> SSVVVDTNGQPVSNGADAYYLVPVSHGHAGLALAKIGNEAEPRAVVLDPHHRPGLPVRFESPLRINIIKESYFLNIKFGPSSSDSGVWDVI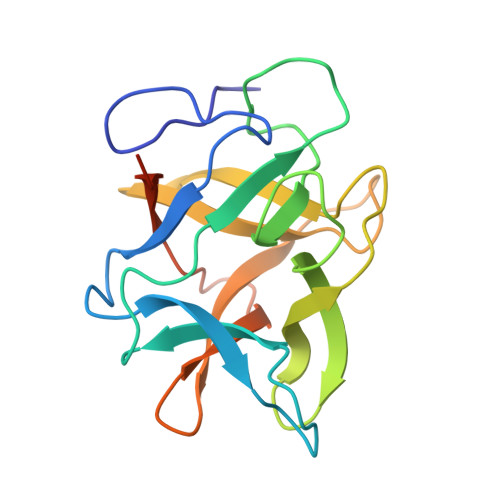QQDPIGLAVKVTDTKSLLGPFKVEKEGEGYKIVYYPERGQTGLDIGLVHRNDKYYLAVKDGEPCVFKIRKATDEESFAGIMSIV>SEYRVDLVVLSEQKQNCRFGLTFHNLSDQDLNSWGLTFAFDRYILPDS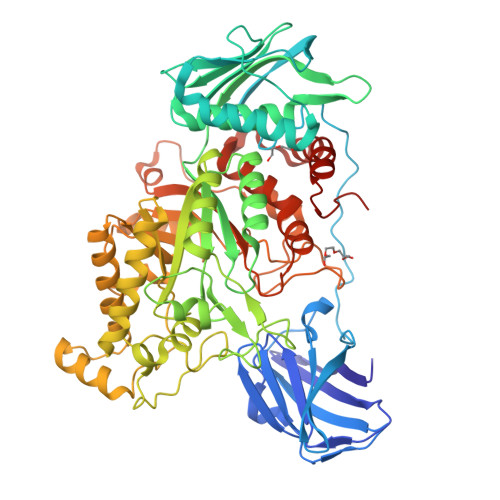VSNGQLTQIGSFCTLKPEGIVLAANHHYYCEFSIGSNPFRYYSDGFNEAMIDFVVDGQPQRAQVDVTPIVLASPYRERSDIPASLTHAQPLLPKPNHIEVSDHSFTFDEQAGVAIYTDLANSAKAWLLEELQRIHQFTLSSSNSGKIIFKSNPTLDEGAYKLKVSEESIKIEAGSSSGFTHACATLLQLLKRDEATKTMEAVCCSIIDSPRFRYRGMMLDCARHFHSVEQVKRLINLLAHYKLNTFHWHLTDDEGWRVEIKSLPQLTEIGAWRGIDETIEPQYTHLSQRYGGFYTQEEIRDVIAFAEQRGITIIPEIDVPGHCRAAIKSLPHLLIEAEDTTEYRSIQHYNDNVINPALPGSYEFIDKVLEEIAALFPAPYVHIGAAEVPNGVWSKSPACQALMEQLGYTDYKELQGHFLRHAEDKLRKLGKRMLGWEEAQHGNKVSKDTVIYSWLSEEAALNCARQGFDVVLQPAQTTYLDMTQDYAPEEPGVDWANPLPLEKAYNYEPLAEVPADDPIRKRIWGIQTALWCEIINNPSRMDYMIFPRLTAMAEACWTEKQHRDWTDYLSRLKGHLPLLDLQGVNYRKPWKRSRSHHHHHH[2x]>[4x]ETAIPFSRRRMPYSLGTDKLEKVDPDKIKSKLSEDVERKLETDMRELYDRLLPTEAIEVNRRELVSKLERLFNTEWPGHDIRVHLFGSSGNLLCSDDSDVDICITTPWRELESVCMIAELLDRHGMEKVVCVSSAKVPIVKIWDPELKLACDMNVNNTLALENTRMVRTYVSIDDRVRPLAMIIKYWTRRRVVNDAAF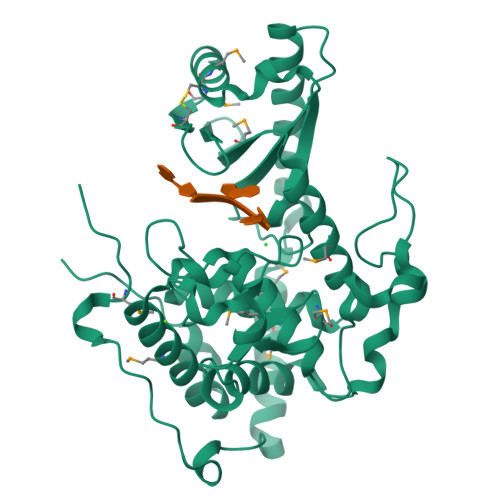GGTLSSYTWICMIIAFLQLRDPPVLPALHQQHDLKLVKQDGALSDFADDIPKLRGFGAKNKDSLAVLLFQFFRFYAHEFDYDKYTLSIRMGTLLTKAEKNWQYLVNNALCVEEPFNDGRNLGNTADETSFRGLHMELRRAFDLIAEGKLEECCEQYVFPKEEERV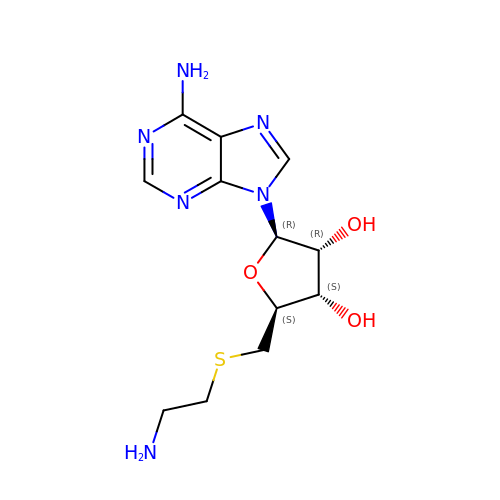5'-DEOXY-5'-[2-(AMINO)ETHYLTHIO]ADENOSINE | C12 H18 N6 O3 S | APAPOJUCRZTCHD-WOUKDFQISA-N In this study, we demonstrate that Flotillin1 and Flotillin2 coassemble to form a large, truncated cone-shaped cage whose wide end is always attached to a membrane surface and whose narrow end is sometimes attached to a separate membrane. The entire wall of the cage is without holes and is likely impervious even to small molecules, forming a diffusion barrier that can connect membrane systems. The Flotillin cage is thus well suited to isolate biochemical processes. Through membrane attachment, it also alters local membrane curvature, which could influence endocytic and mechanosensory processes.

We conclude that the cage consists predominantly of 22 each of Flotillin1 and Flotillin2 in an alternating pattern. With a final density map for the overall Flotillin complex at 3.5 Å resolution, atomic models could be built for much of the molecule. The final model consists of Flotillin-1:1-422 and Flotillin-2:1-402. The wide end has a diameter of 32 nm, the narrow end 19 nm, and height 22 nm. The wide end contains SPFH1 and SPFH2 domains at the N terminus. The wall is a single-layered α-helical barrel, and the narrow end consists of the two α-helical layers described above, one with 22 and the other with 44 α-helices. A β-strand from each Flotillin makes a 44-stranded β-barrel inside the helical layer. The narrow end is made by the C terminus of Flotillin arranged in two layers of helices that run in opposite directions and are linked by a β-strand. Adherence to the membrane is mediated by the SPFH1 domains, which penetrate one leaflet of the lipid bilayer. The Flotillin cage, by contrast, uses a hydrophobic surface that contains covalent lipid molecules.

> MGNCHTVGPNEALVVSGGCCGSDYKQYVFGGWAWAWWCISDTQRLSLEVMTILCRCENIETSEGVPLFVTGVAQVKIMTEKELLAVACEQFLGKNVQDIKNVVLQTLEGHLRSILGTLTVEQIYQDRDQFAKLVREVAAPDVGRMGIEILSFTIKDVYDKVDYLSSLGKTQTAVVQRDADIGVAEAERDAGIREAECKKEMLDVKFMADTKIADSKRAFELQKSAFSEEVNIKTAEAQLAYELQGAREQQKIRQEEIEIEVVQRKKQIAVEAQEILRTDKELIATVRRPAEAEAHRIQQIAEGEKVKQVLLAQAEAEKIRKIGEAEAAVIEAMGKAEAERMKLKAEAYQKYGDAAKMALVLEALPQIAAKIAAPLTKVDEIVVLSGDNSKVTSEVNRLLAEL;> MFFTCGPNEAMVVSGFCRSPPVMVAGGRVFVLPCIQQIQRISLNTLTLNVKSEKVYTRHGVPISVTGIAQVKIQGQNKEMLAAACQMFLGKTEAEIAHIALETLEGHQRAIMAHMTVEEIYKDRQKFSEQVFKVASSDLVNMGISVVSYTLKDIHDDQDYLHSLGKARTAQVQKDARIGEAEAKRDAGIREAKAKQEKVSAQYLSEIEMAKAQRDYELKKAAYDIEVNTRRAQADLAYQLQVAKTKQQIEEQRVQVQVVERAQQVAVQEQEIARREKELEARVRKPAEAERYKLERLAEAEKSQLIMQAEAEAASVRMRGEAEAFAIGARARAEAEQMAKKAEAFQLYQEAAQLDMLLEKLPQVAEEISGPLTSANKITLVSSGSGTMGAAKVTGEVLDILTRLPESVERLTGVSISQVNHK>[2x]MLVLVIGDFHVPHRSAAIPQVFLDRLNTGRIQTVLCTGNLCGKETYDILRTLAREVHVVKGAFDEMQG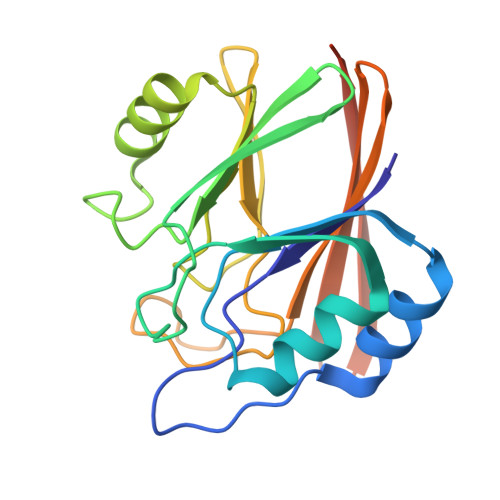LNETEVIKIGNFKIGLMAGHQVIPWGDREALAIYQRQLDVDILITGHTHKLETKEVGGKYFLNPGSATGAYSPLVDNPVPSFMLLEINDSELTIYEYTLVDGSVKCERVDFNKKQQQLEHHHHHH> AEMKSRYTTEFHELEKIGSGEFGSVFKCVKRLDGCIYAIKRSKKPLAGSVDEQNALREVYAHAVLGQHSHVVRYFSAWAEDDHMLIQNEYCNGGSLADAISENYRIMSYFKEAELKDLLLQVGRGLRYIHSMSLVHMDIKPSNIFISRTSIPNAASEEGDEDDWA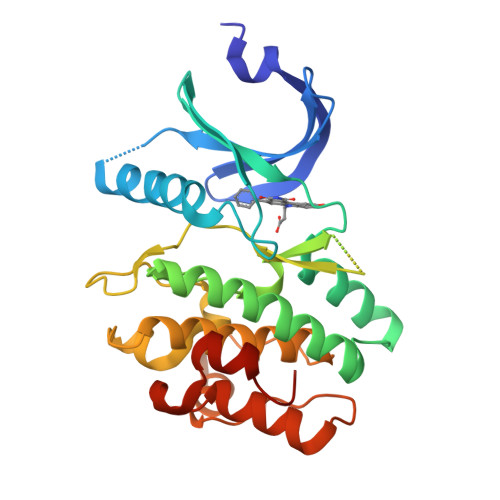SNKVMFKIGDLGHVTRISSPQVEEGDSRFLANEVLQENYTHLPKADIFALALTVVCAAGAEPLPRNGDQWHEIRQGRLPRIPQVLSQEFTELLKVMIHPDPERRPSAMALVKHSVLLSASRK Many streptococci adhere to protein-attached carbohydrates expressed on cell surfaces using Siglec-like binding regions (SLBRs). Siglec-like binding regions (SLBRs) are among the streptococcal adhesive modules that bind sialoglycans. SLBRs contain two adjacent modules: a Siglec domain, which shares some features with mammalian Siglecs, and a Unique domain13 with no close homologs outside of the family. The conserved sialic acid-recognition motif governs general specificity while sequence diversity in surrounding loop regions allows the SLBR to select between related sialoglycans.

SLBRGspB exhibits narrow specificity for the sTa trisaccharide, as have other previously-characterized members of this evolutionary branch. To reveal how similar SLBRs could include or exclude different sialoglycans, we determined crystal structures of these five SLBRs at resolutions between 1.0 Å and 1.7 Å. This included a structure of SLBRGspB with improved resolution as compared to a previous report. Finally, molecular dynamics (MD) simulations of unliganded SLBRHsa and SLBRGspB predict that these loops exhibit considerably more flexibility than other parts of the protein.

> SDTERPVVNVPSEITVYRGESFEYFATVTDNSNAFDLAKTVVRWLYSNQPGRGTEWLQYSVTQVGNQLKVRIFGNVPIDTTIGDYTRYVVATDAAGNVNATQTEMGNAAVDKTSVNGQFKLIIRFRIKTPENTVFVNNPNQLTEVEKNLVREAVKKSNPDLRAQDVLNSNYVTGITVSNNGTTTITYRDGRKDIIDGSKFIDTR>GSEELLDLFNRQVTQEFTASQVYLSASIWFDQNDWEGMAAYMLAESAEEREHGLGFVDFANKRNIPIELQAVPAPVSCAEW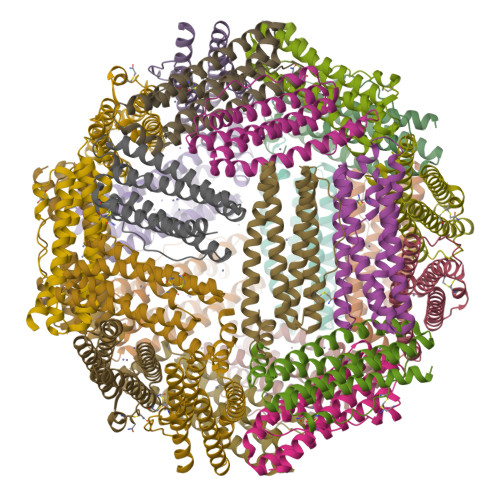SSPEDVWQSILELEQANTRSLLNLAEAASTCHDFAVMAFLNPFHLQQVNEEDKIGSILAKVTDENRTPGLLRSLDVVSFLGPCLFRS[8x]>ME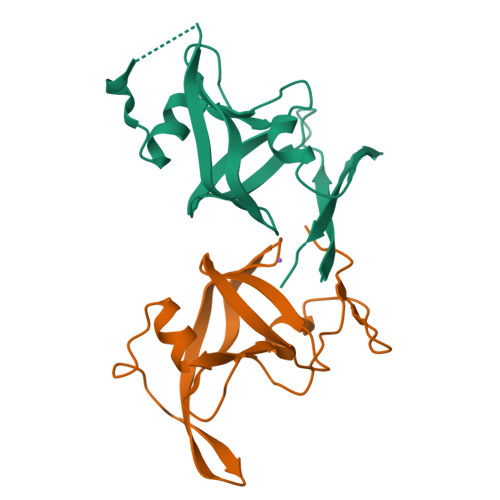VGEIIIARNRDGHFYINAFVNNVKIKFMVDTGASDIALTKEDAQKLGFDLTKLKYTRTYLTANGENKAAPITLNSVVIGKEFKNIKGHVGLGDLDISLLGMSLLERFKGFRIDKDLLILNYAAALEHHHHHH[2x]> HHHHHHMFGQLTGGLEAAWSKLKGEEVLTKDNIAEPMRDIRRALLEADVSLPVVRRFVQSVSDQAVGMGVIRGVKPDQQLVKIVHDELV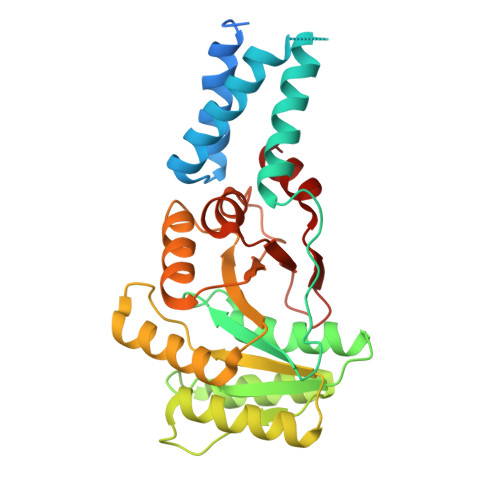KLMGGEVSELQFAKSGPTVILLAGLQGVGKTTVCAKLACYLKKQGKSCMLIAGDVYRPAAIDQLVILGEQVGVPVYTAGTDVKPADIAKQGLKEAKKNNVDVVIMDTAGRLQIDKGMMDELKDVKKFLNPTEVLLVVDAMTGQEAAALVTTFNVEIGITGAILTKLDGDSRGGAALSVKEVSGKPIKLVGRGERMEDLEPFYPDRMAGRILG> MRNPFERMPTVLTADELIDKAFRRAEKAASSFKPRGNKVKKARLREELRVRTVSNVVRDNLRKVLERTPGLSTLPKFYQELVDVLVDRDTFHKAMAGIDWAIRIIRELEERYVERIRYSNDPNEIAELRRQFYGRVASVLRDIDDRLRYLNKAREVLKDLPVVDLEIPTVVIAGHPNVGKSTLLKALTTAKPEIASYPFTTRGINVGQFEDGYFRYQIIDTPGLLDRPISERNEIEKQAILALRYLGNLIIYIFDPSEHCGFPLEEQIHLFEEVHGEFKDLPFLVVINKIDVADEENIK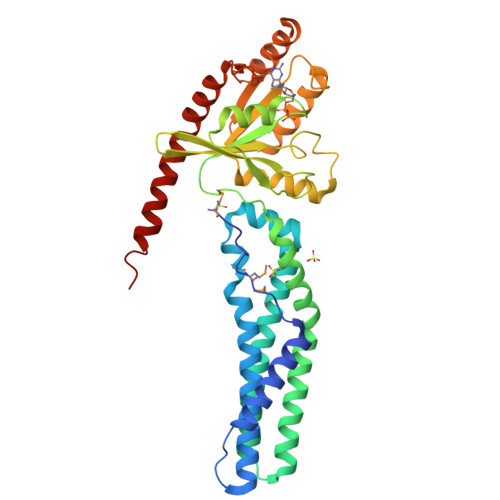RLEKFVKEKGLNPIKISALKGTGIDLVKEEIIKTLRPLAEKVAREKIERELRRYRSYL>[6x]EV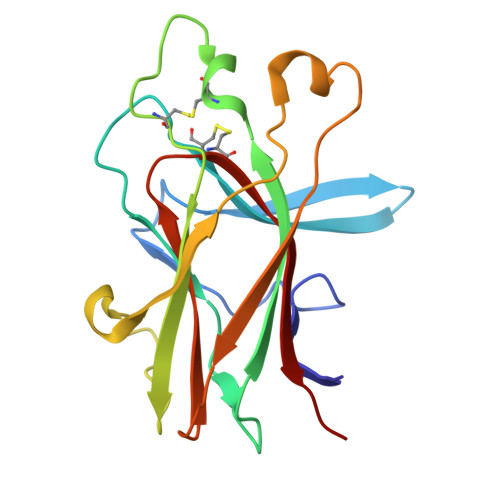VLLDFAAAGGELGWLTHPYGKGWDLMQNIMNDMPIYMYSVCNVMSGDQDNWLRTNWVYRGEAERIFIELKFTVRDCNSFPGGASSCKETFNLYYAESDLDYGTNFQKRLFTKIDTIAPDEITVSSDFEARHVKLNVEERSVGPLTRKGFYLAFQDIGACVALLSVRVYYKKC> 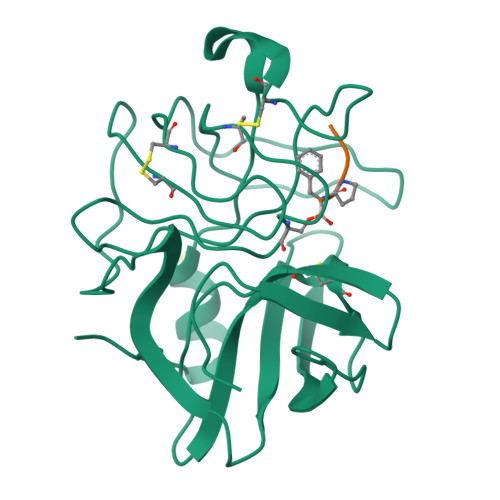ANIVGGIEYSINNASLCSVGFSVTRGATKGFVTAGHCGTVNATARIGGAVVGTFAARVFPGNDRAWVSLTSAQTLLPRVANGSSFVTVRGSTEAAVGAAVCRSGRTTGYQCGTITAKNVTANYAEGAVRGLTQGNACMGRGDSGGSWITSAGQAQGVASGGNVQSNGNNCGIPASQRSSLFERLQPILSQYGLSLVTG;> XAAPF> MKTKPLPTAPMAWAESAVETTTSPRELAGHAPLRRVLRPPIARRDGPVLLGDRAPRRTASTMWLLGIDPAESSPGTRATRDDTEQAVDKILRGARRAGGLTVPGAPRYHLTRQVTLTDLCQPNAERAGALLLALRHPTDLPHLARHRAPPGRQTERLAEAWGQLLEASALGSGRAESGCARAGLVSFNFLVAACTAAYDARDAAEAVRAHITTNYGGTRAGARLDRFS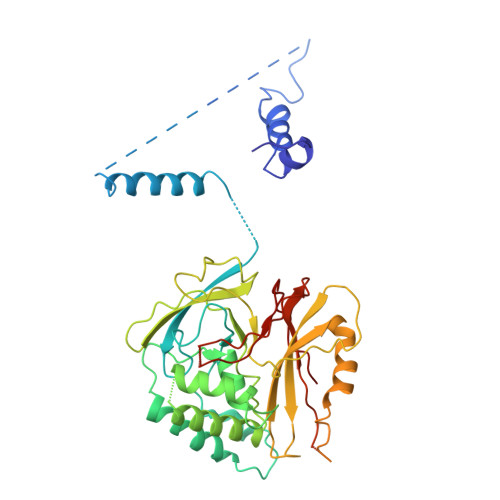ECLRAMVHTHVFPHEVMRFFGGLVSWVTQDELASVTAVCSGPQEATHTGHPGRPCSAVTIPACAFVDLDAELCLGGPGAAFLYLVFTYRQCRDQELCCVYVVKSQLPPRGLEAALERLFGRLRITNTIHGAEDMTPPPPNRNVDFPLAVLAASSQSPRCSASQVTNPQFVDRLYRWQPDLRGRPTARTCTYAAFAELGVMPDDSPRCLHRTERFGAVGVPVVILEGVVWRPGGWRACA>MKFFSYILVYRRFLFVVFTVLVLLPLPIVLHTKEAECAYTLFVVATFWLTEALPLSVTALLPSLMLPMFGIMPSKKVASAYFKDFHLLLIGVICLATSIEKWNLHKRIALKMVMMVGVNPAWLTLGFMSSTAFLSMWLSNTSTAAMVMPIAEAVVQQIINAEAEVEATQMTYFNGSTNHGLEIDESVNGHEINERKEKTKPVPGYNNDTGKISSKVELEKNSGMRTKYRTKKGHVTRKLTCLCIAYSSTIGGLT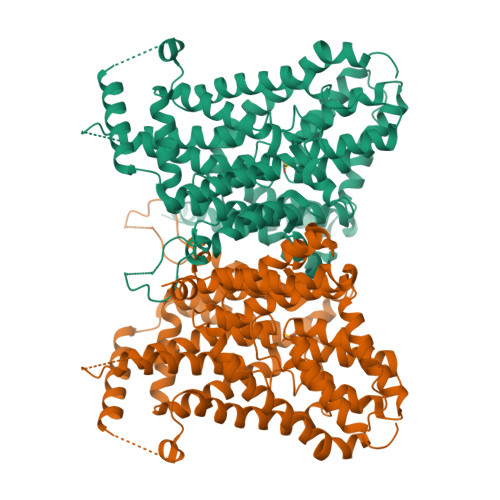TITGTSTNLIFAEYFNTRYPDCRCLNFGSWFTFSFPAALIILLLSWIWLQWLFLGFNFKEMFKCGKTKTVQQKACAEVIKQEYQKLGPIRYQEIVTLVLFIIMALLWFSRDPGFVPGWSALFSEYPGFATDSTVALLIGLLFFLIPAKTLTKTTPTGEIVAFDYSPLITWKEFQSFMPWDIAILVGGGFALADGCEESGLSKWIGNKLSPLGSLPAWLIILISSLMVTSLTEVASNPATITLFLPILSPLAEAIHVNPLYILIPSTLCTSFAFLLPVANPPNAIVFSYGHLKVIDMVKAGLGVNIVGVAVVMLGICTWIVPMFDLYTYPSWAPAMSNETMP[2x]4'-EPIDOXORUBICIN | C27 H30 N O11 | 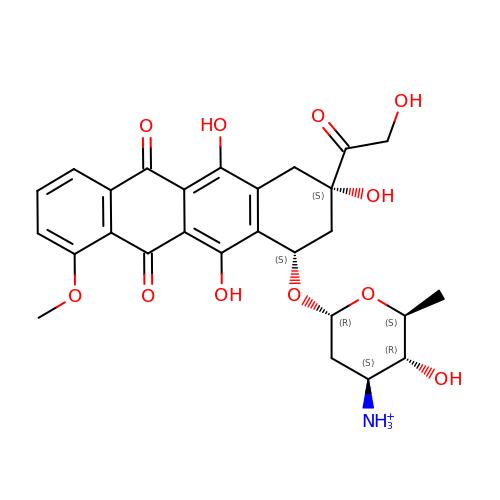AOJJSUZBOXZQNB-VTZDEGQISA-O(3~{a}~{S},8~{a}~{S})-6-(phenylcarbonyl)-2,3,3~{a},7,8,8~{a}-hexahydropyrrolo[3,4-d]azepin-1-one | C15 H16 N2 O2 | 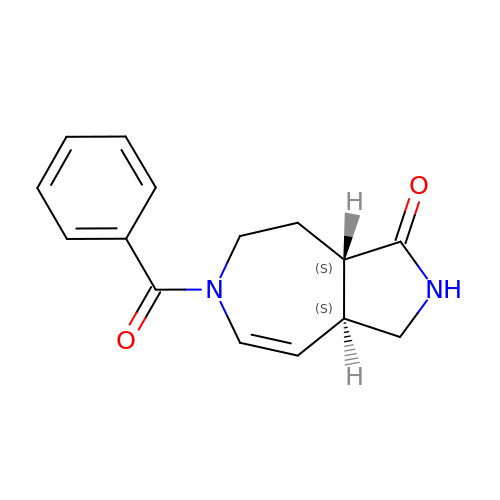KCUQXPDGHOUBAD-OLZOCXBDSA-N> GEGMWVPQQLPEIAGPLKKAGLKLSPQQISDLTGDPMGAVVALGGCTASFVSPNGLVVTNHACAYGAIQLNSTAENNLIKNGFNAPTTADEVSAGPNARVFVLDEITDVTKDAKAAIAAAGDDALARTKALEAFEKKLIADCEAEAGFRCRLYSFSGGNTYRLFKNLEIKDVRLAYAPPGSVGKFGGDIDNWMWPRHTGAFAFYRAYVGKDGKPAAFSKDNVPYQPKHWLKFADQPLGAGDFVMVAGYPGSTNRYALAAEFDNTAQWTYPTIARHYKNQIAMVEAAGKQNADIQVKYAATMAGWNNTSKNYDGQLEGFKRIDAAGQKLREEAAVLGWLKGQGAKGQPALDAHAKLLDLLEQSKATRDRDLTLALFNNTAMLGSATQLYRLSIEREKPNAERESGYQERDLPAIEGGLKQLERRYVAAMDRQLQEYWLNEYIKLPADQRVAAVDAWLGGNDAAAVKRALDRLAGTKLGSTEERLK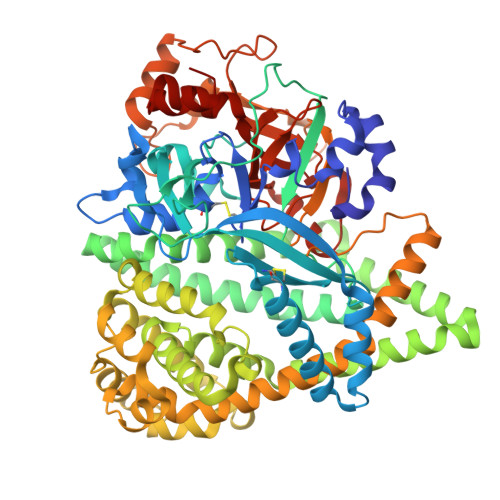WFAADRKAFEASNDPAIQYAVAVMPTLLKLEQERKTRAGENLAARPVYLQALADYKKSQGEFVYPDANLSLRITFGNVMGYAPKDGMEYTPFTTLEGVVAKETGQDPFDSPKALLDAVAAKRYGGLEDKRIGSVPVNYLSDLDITGGNAGSPVLDAHGKLVGLAFDGNWESVSSNWVFDPKMTRMIAVDGRYLRWIMQEVYPAPQLLKEMNVGK> MNDIAHNLAQVRDKISAAATRCGRSPEEITLLAVSATKPASAIAEAIDAGQRQFGENYVQEGVDKIRHFQELGVTGLEWHFIGPLQSNKSRLVAEHFDWCHTIDRLRIATRLNDQRPAELPPLNVLIQINISDENSKSGIQLAELDELAAAVAELPRLRLRGLMAIPAPESEYVRQFEVARQMAVAFAGLKTRYPHIDTLSLGMSDDMEAAIAAGSTMVRIGTAIFGARDYS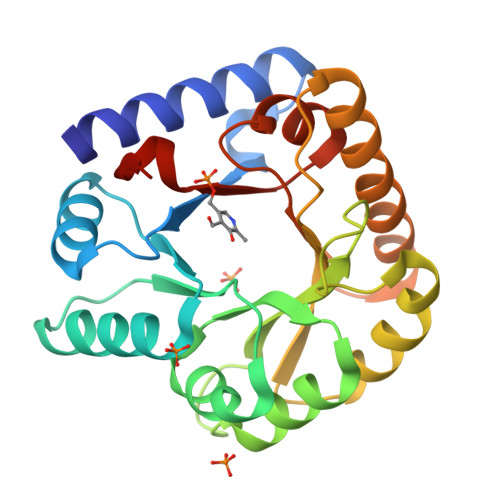KK> MGSDKIHHHHHHMITTTIFPGRYVQGAGAINILEEELSRFGERAFVVIDDFVDKNVLGENFFSSFTKVRVNKQIFGGECSDEEIERLSGLVEEETDVVVGIGGG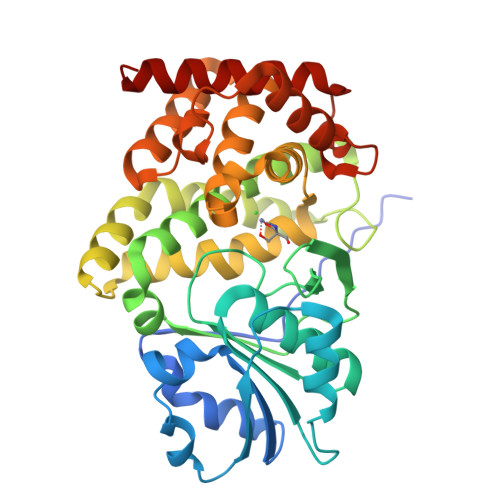KTLDTAKAVAYKLKKPVVIVPTIASTDAPCSALSVIYTPNGEFKRYLFLPRNPDVVLVDTEIVAKAPARFLVAGMGDALATWFEAESCKQKYAPNMTGRLGSMTAYALARLCYETLLEYGVLAKRSVEEKSVTPALEKIVEANTLLSGLGFESGGLAAAHAIHNGLTVLENTHKYLHGEKVAIGVLASLFLTDKPRKMIEEVYSFCEEVGLPTTLAEIGLDGVSDEDLMKVAEKACDKNETIHNEPQPVTSKDVFFALKAADRYGRMRKNLT> IESIIKTATDTVKSEINAELGVVPSLNAVETGATSNTEPEEAIQTRTVINQHGVSETLVENFLSRAALVSKRSFEYKDHTSSTAQTDKNFFKWTINTRSFVQLRRKLELFTYLRFDAEITILTTVAVNGSNNNTYVGLPDLTLQAMFVPTGALTPEKQDSFHWQSGSNASVFFKISDPPARMTIPFMCINSAYSVFYDGFAGFEKTGLYGINPADTIGNLCVRIVNEHQPVGFTVTVRVYMKPKHIKAWAPRPPRTLPYMSIANANYKGKERAPNALNAIIGNRDSVKTMPHNIV;> SPSAEACGYSDRVLQLKLGNSAIVTQEAANYCCAYGEWPNYLPDHEAVAIDKPTQPETATDRFYTLRSVKWEATSTGWWWKLPDALNNIGMFGQNVQHHYLYRSGFLIHVQCNATKFHQGALLVVAIPEHQRGAHNTTTSPGFDDIMKGEAGGTFNHPYVLDDGTSLACATIFPHQWINLRTNNSATIVLPWMNAAPMDFPLRHNQWTLAIIPVVPLGTRTMSSMVPITVSIAPMCCEFNGLRHAITQ;> GVPTYLLPGSGQFLTTDDHSSAPVLPCFNPTPEMHIPGQVRNMLEVVQVESMMEINNTESAVGMERLKVDISALTDVDQLLFNIPLDIQLDGPLRNTLVGNISRYYTHWSGSLEMTFMFCGSFMATGKLILCYTPPGGSCPTTRETAMLGTHIVWDF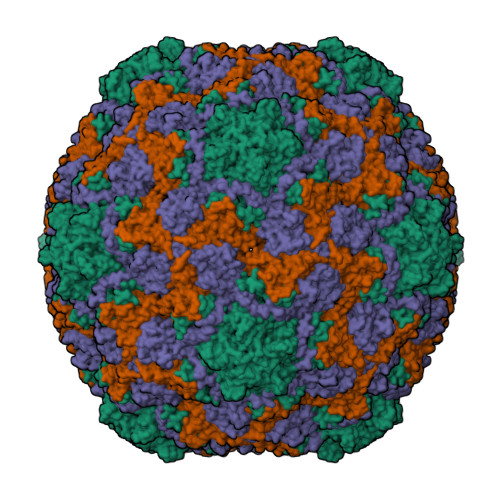GLQSSITLIIPWISGSHYRMFNNDAKSTNANVGYVTCFMQTNLIVPSESSDTCSLIGFIAAKDDFSLRLMRDSPDIGQIDHLHGAEAAYQ We introduce the spitrobot, a protein crystal plunger, enabling reaction quenching via cryo-trapping with a time-resolution in the millisecond range. Protein crystals are mounted on canonical micromeshes on an electropneumatic piston, where the crystals are kept in a humidity and temperature-controlled environment, then reactions are initiated via the liquid application method (LAMA) and plunging into liquid nitrogen is initiated after an electronically set delay time to cryo-trap intermediate states. Traditionally cryo-trapping has been exploited to quench enzymatic reactions within protein crystals and thereby obtain structural information about reaction intermediates.

We also trap reaction intermediates and conformational changes in macroscopic crystals of tryptophan synthase to demonstrate that the spitrobot enables insight into catalytic events. By contrast, the spitrobot is built around the SPINE-standard, and versatile time delays have been demonstrated. While true time-resolved crystallographic experiments at room temperature offer a much more complete access to the dynamic landscape of protein function, cryo-trapping experiments may be sufficient to solve many important biologically relevant questions—e.g., provide insight into thermodynamically trapped, stable reaction intermediates. It is clear that care has to be taken to only use crystals of highly similar dimensions to avoid that mechanistic conclusions are affected by different diffusion times.

> HMERYENLFAQLNDRREGAFVPFVTLGDPGIEQSLKIIDTLIDAGADALELGVPFSDPLADGPTIQNANLRAFAAGVTPAQCFEMLALIREKHPTIPIGLLMYANLVFNNGIDAFYARCEQVGVDSVLVADVPVEESAPFRQAALRHNIAPIFICPPNADDDLLRQVASYGRGYTYLLSRSGVTGAENRGALPLHHLIEKLKEYHAAPALQGFGISSPEQVSAAVRAGAAGAISGSAIVKIIEKNLASPKQMLAELRSFVSAMKAASRA;> MTTLLNPYFGEFGGMYVPQILMPALNQLEEAFVSAQKDPEFQAQFADLLKNYAGRPTALTKCQNITAGTRTTLYLKREDLLHGGAHKTNQVLGQALLAKRMGKSEIIAETGAGQHGVASALASALLGLKCRIYMGAKDVERQSPNVFRMRLMGAEVIPVHSGSATLKDACNEALRDWSGSYETAHYMLGTAAGPHPYPTIVREFQRMIGEETKAQILDKEGRLPDAVIACVGGGSNAIGMFADFINDTSVGLIGVEPGGHGIETGEHGAPLKHGRVGIYFGMKAPMMQTADGQIEESYSISAGLDFPSVGPQHAYLNSIGRADYVSITDDEALEAFKTLCRHEGIIPALESSHALAHALKMMREQPEKEQLLVVNLSGRGDKDIFTVHDILKARGEI> KPRGKRGWLWLLLKLAIVFAVLIAIYGVYLDQKIRSRIDGKVWQLPAAVYGRMVNLEPDMTISKNEMVKLLEATQYRQVSKMTRPGEFTVQANSIEMIRRPFDFPDSKEGQVRARLTFDGDHLATIVNMENNRQFGFFRLDPRLITMISSPNGEQRLFVPRSGFPDLLVDTLLATEDRHFYEHDGISLYSIGRAVLANLTAGRTVQGASTLTQQLVKNLFLSSERSYWRKANEAYMALIMDARYSKDRILELYMNEVYLGQSGDNEIRGFPLASLYYFGRPVEELSLDQQALLVG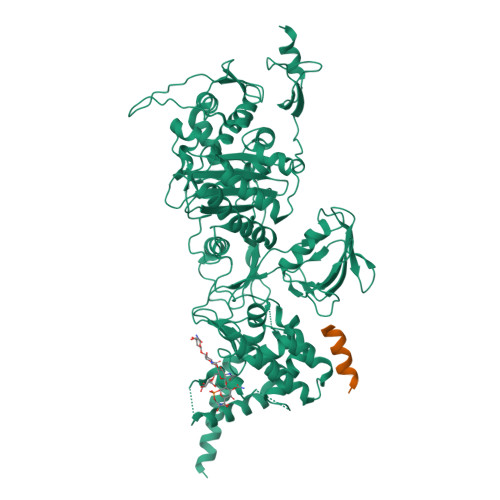MVKGASIYNPWRNPKLALERRNLVLRLLQQQQIIDQELYDMLSARPLGVQPRGGVISPQPAFMQLVRQELQAKLGDKVKDLSGVKIFTTFDSVAQDAAEKAAVEGIPALKKQRKLSDLETAIVVVDRFSGEVRAMVGGSEPQFAGYNRAMQARRSIGSLAKPATYLTALSQPKIYRLNTWIADAPIALRQPNGQVWSPQNDDRRYSESGRVMLVDALTRSMNVPTVNLGMALGLPAVTETWIKLGVPKDQLHPVPAMLLGALNLTPIEVAQAFQTIASGGNRAPLSALRSVIAEDGKVLYQSFPQAERAVPAQAAYLTLWTMQQVVQRGTGRQLGAKYPNLHLAGKTGTTNNNVDTWFAGIDGSTVTITWVGRDNNQPTKLYGASGAMSIYQRYLANQTPTPLNLVPPEDIADMGVDYDGNFVCSGGMRILPVWTSDPQSLCQQSEMQQQPS;> LPPKPEERWRYIKELESRQ> IVGGFKCEKNSQPWHVAVYRYTQYLCGGVLLDPNWVLTAAHCYDDNYKVWLGKNNLFKDEPSAQHRFVSKAIPHPGFNMSLMRKHIRFLEYDYSNDLMLLRLSKPADITDTVKPITLPTEEPKLGSTCLASGWGSITPTKFQFTDDLYCVNLKLLPNEDCAKAHIEKVTDAMLCAGEMDGGKDTCKGDSGGPLICDGVLQG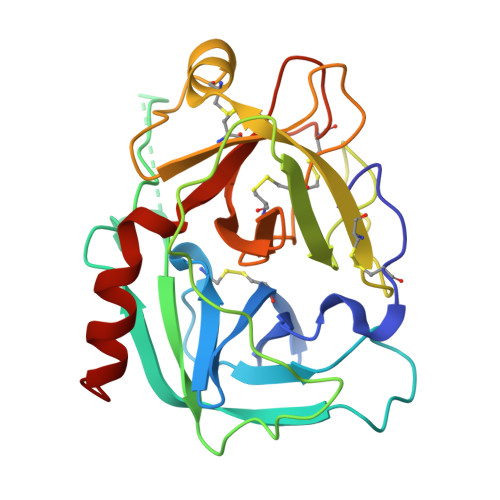ITSWGHTPCGEPDMPGVYTKLNKFTSWIKDTMAKNP> DPEK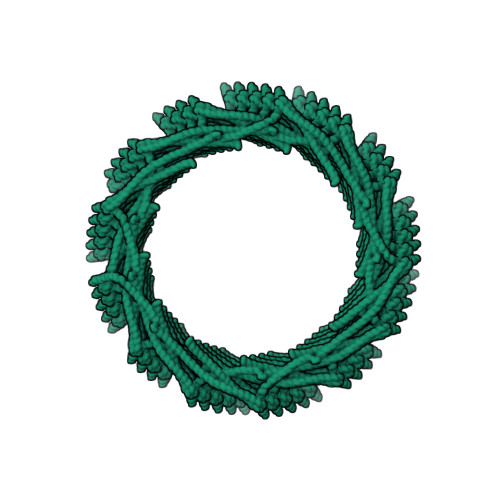VLEQAVIDMQEDLVQLRQAVARTIAEEKRTEQRLNQDTQEAKKWEDRAKLALTNGEENLAREALARKKSLTDTAAAYQTQLAQQRTMSENLRRNLAALEAKISEAKTKKNMLQARAKAAKANAELQQTLGGLGTSSATSAFERMENKVLDMEATSQAAGELAGFGIENQFAQLEASSGVEDELAALKA> MPITINNFNYSDPVDNKNILYLDTHLNTLANEPEKAFRITGNIWVIPDRFSRNSNPNLNKPPRVTSPKSGYYDPNYLSTDSDKDTFLKEIIKLFKRINSREIGEELIYRLSTDI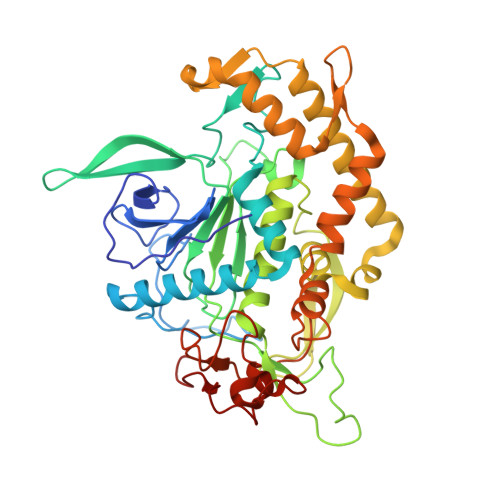PFPGNNNTPINTFDFDVDFNSVDVKTRQGNNWVKTGSINPSVIITGPRENIIDPETSTFKLTNNTFAAQEGFGALSIISISPRFMLTYSNATNDVGEGRFSKSEFCMDPILILMHELNHAMHNLYGIAIPNDQTISSVTSNIFYSQYNVKLEYAEIYAFGGPTIDLIPKSARKYFEEKALDYYRSIAKRLNSITTANPSSFNKYIGEYKQKLIRKYRFVVESSGEVTVNRNKFVELYNELTQIFTEFNYAKIYNVQNRKIYLSNVYTPVTANILDDNVYDIQNGFNIPKSNLNVLFMGQNLSRNPALRKVNPEPLV> SNAMHIKSAIIVVSDRISTGTRENKALPLLQRLMSDELQDYSYELISEVVVPEGYDTVVEAIAT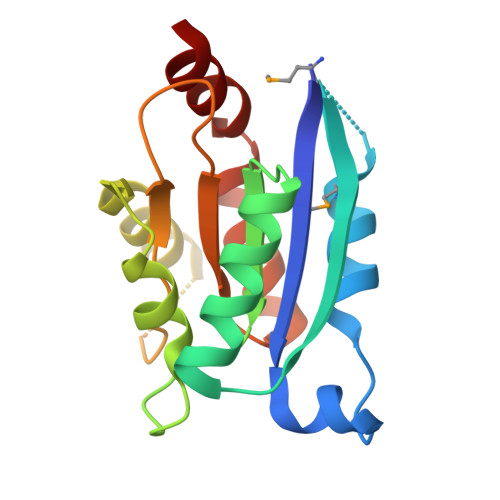ALKQGARFIITAGGTGIRAKNQTPEATASFIHTRCEGLEQQILIHGSTHTHLAGLSRGIVGVTGRDDHAALIVNAPSSSGGITDTWAVISPVIPNIFEGLDAS> MGALEELRGQY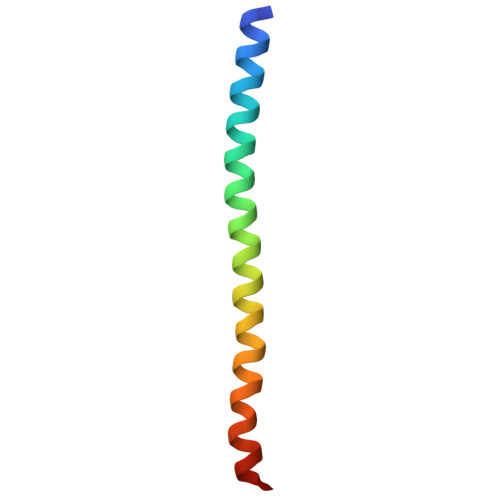IKAVKKIKCDMLRYIQESKERAAEMVKAEVLRERQETARKMRK> PRKKK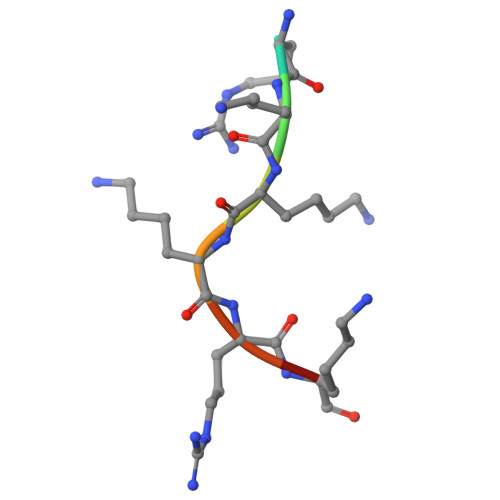RKH> ESKSYGSG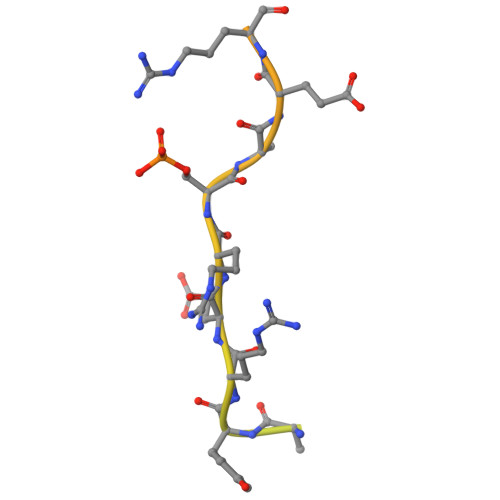SRRERSRERDHSRSREKSRRHKSRSRDRHDDYYRERSRERERHRDRDRDRDRERDREREYRH>[2x]GPAAAEPRPTAPSSGAPGLAGVGETPSAAALAAARVELPGTAVPSVPEDAAPASRDGGGVRDEGPAAAGDGLGRPLGPTPSQSRFQVDLVSENAGRAAAAAAAAAAAAAAAGAGAGAKQTPADGEASGESEPAKGSEEAKGRFRVNFVDPAASSSAEDSLSDAAGVGVDGPNVSFQNGGDTVLSEGSSLHSGGGGGSGHHQHYYYDTHTNTYYLRTFGHNTMDAVPRIDHYRHTAAQLGEKLLRPSLAELHDELEKEPFEDGFANGEESTPTRDAVVTYTAESKGVVKFGWIKGVLVRCMLNIWGVMLFIRLSWIVGQAGIGLSVLVIMMATVVTTITGLSTSAIATNGFVRGGGAYYLISRSLGPEFGGAIGLIFAFANAVAVAMYVVGFAETVVELLKEHSILMIDEINDIRIIGAITVVILLGISVAGMEWEAKAQIVLLVILLLAIGDFVIGTFIPLESKKPKGFFGYKSEIFNENFGPDFREEETFFSVFAIFFPAATGILAGANISGDLADPQSAIPKGTLLAILITTLVYVGIAVSVGSCVVR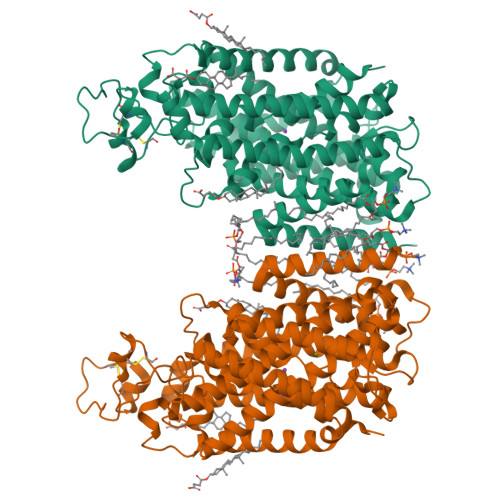DATGNVNDTIVTELTNCTSAACKLNFDFSSCESSPCSYGLMNNFQVMSMVSGFTPLISAGIFSATLSSALASLVSAPKIFQALCKDNIYPAFQMFAKGYGKNNEPLRGYILTFLIALGFILIAELNVIAPIISNFFLASYALINFSVFHASLAKSPGWRPAFKYYNMWISLLGAILCCIVMFVINWWAALLTYVIVLGLYIYVTYKKPDVNWGSSTQALTYLNALQHSIRLSGVEDHVKNFRPQCLVMTGAPNSRPALLHLVHDFTKNVGLMICGHVHMGPRRQAMKEMSIDQAKYQRWLIKNKMKAFYAPVHADDLREGAQYLMQAAGLGRMKPNTLVLGFKKDWLQADMRDVDMYINLFHDAFDIQYGVVVIRLKEGLDISHLQGQEELLSSQEKSPGTKDVVVSVEYSKKSDLDTSKPLSEKPITHKVEEEDGKTATQPLLKKESKGPIVPLNVADQKLLEASTQFQKKQGKNTIDVWWLFDDGGLTLLIPYLLTTKKKWKDCKIRVFIGGKINRIDHDRRAMATLLSKFRIDFSDIMVLGDINTKPKKENIIAFEEIIEPYRLHEDDKEQDIADKMKEDEPWRITDNELELYKTKTYRQIRLNELLKEHSSTANIIVMSLPVARKGAVSSALYMAWLEALSKDLPPILLVRGNHQSVLTFYS>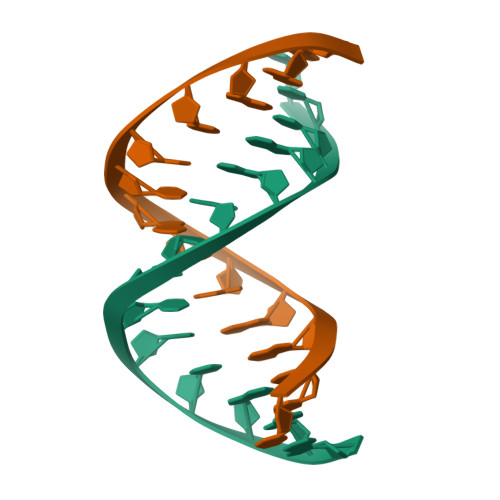CCCGGGTACCCGGG[2x]> GAMGPTSNDACLSIVHSLMCHRQGGESETFAKRAIESLVKKLKEKKDELDSLITAITTNGAHPSKCVTIQRTLDGRLQVAGRKGFPHVIYARLWRWPDLHKNELKHVKYCQYAFDLKCDSVCVNPYHYERVVSPG

Smad proteins consist of an N-terminal MH1 domain, which binds to DNA, a linker region with phosphorylation sites for network regulatory inputs, and a C-terminal MH2 domain that is phosphorylated by the receptors and binds other Smad proteins, LDTFs, chromatin readers, and transcriptional co-activators and co-repressors. The receptors for TGF-β, nodal, activin, myostatin, and other family members are membrane serine/threonine kinases that phosphorylate and activate Smad2 and Smad3, whereas analogous receptors for the bone morphogenetic proteins (BMPs) preferentially phosphorylate and activate Smads 1, 5, and 8. These receptor-activated Smads (R-Smads) form heterotrimeric complexes with Smad4, which is required for the transcriptional regulation of most target genes. Focusing on the human and mouse Gsc promoter, here we identify specific Smad-binding GC-rich motifs and provide the X-ray crystal structures of Smad3 and Smad4 bound to several of these motifs. The structures determined here reveal that the β-hairpin is flexible and adaptable to bind with high-affinity several variants of the consensus sequence GGC(GC)|(CG), which we refer to as 5GC SBE.

The best diffracting crystals were obtained with DNAs of 16 and 18 bp. A complex with the 18 bp dsDNA oligonucleotide containing the GGCGCG sequence from the GC1 Gsc segment yielded data at 2.05 Å (refer to Methods section and Table 1). In the complex, the convex face of the DNA-binding hairpin dives into the concave major groove of the duplex DNA containing five base pairs (6-GGCGC-10/9′-GCGCC-13′). In the complex with the 6-GGCGCG-11 site, these three residues also participate in a network of hydrogen bonds with the first four consecutive base pairs of the GGCGC motif. Specifically, the guanidine group of Arg81 side chain coordinates tightly the G6 nucleotide. The orientation of Arg81 is further stabilized by the interaction of Asp79 side chain with the guanidine site of Arg81. In addition, Lys88 side chain is also well defined through interactions with both G7 and G11′, the latter being located in the complementary chain. The Gln83 side chain carbonyl interacts with C10′, while the amide part is in the proximity of the C9′ phosphate. The complex is further reinforced by a set of hydrogen bond interactions between the backbones of Leu78, Gln83, and Ala85, with G11, G9′, and C10′, covering the 6-GGCGCG-11 area and by a network of well-ordered water molecules, which are tightly bound at the interface of the protein–DNA-binding site. Ten of the water molecules are closely coordinated by residues of the β2–β3 hairpin and six bases of the GGGCGCGC region. Additionally, five more water molecules strengthen the interactions of the N-terminal helix α2 with the phosphates of the DNA backbone.> GHMMRKLGLIAGGGALPVELASHCEAAGRAFAVMRLRSFADPSLDRYP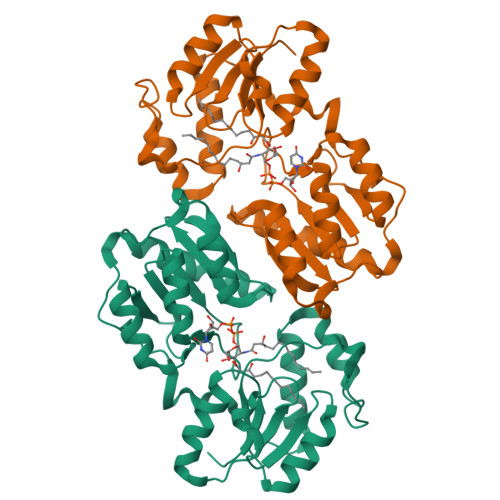GADVGIGEFGKIFKALRAEGCDVVCFAGNVSRPDFSALMPDARGLKVLPSLIVAARKGDDALLRRVLDEFEKEGFEIEGAHEVMGEMTLPRGRLGKVSPAPEHMADIDKALDVAREIGRLDIGQGAVVCEGLVLAVEAQEGTDAMLRRVADLPEAIRGRAERRLGVLAKAPKPIQETRVALPTIGVATIHRAARAGLAGIVGEAGRLLVVDREAVIAAADDLGLFVLGVDPQERP> GPMDFVETNSAVYFYGQRDRKFGFLSNFYPCEFTDTEGRRFYSSEQYFMKRKQEMFDRDNEKVAIAILRAKAPAVAKKLGRQVENYDDEVWAEHRYEVMLEALKLKFSSDEEMAAKLLATGAKRLYEASRHDAIWGIGLSVASVTRMFRESVSFQRTGDVDAETRSLCFGKNLLGNALMEARAWLQPQD

Modification of nucleic acids by ADP-ribosylation is catalyzed by various ADP-ribosyltransferases, including the DarT enzyme. The latter is part of the bacterial toxin-antitoxin (TA) system DarTG, which was shown to provide control of DNA replication and bacterial growth as well as protection against bacteriophages. Using structural and biochemical approaches, we show that DarT1-NADAR is a TA system for reversible ADP-ribosylation of guanosine bases. DarT1 evolved the ability to link ADP-ribose to the guanine amino group, which is specifically hydrolyzed by NADAR.

Furthermore, we support our studies with the first crystal structures of NADARs in their ligand-free and ADPr-bound states to structurally characterize the DarT1-associated BC4488 subfamily NADARs in comparison with orphan YbiA subfamily NADARs using that from the plant-pathogenic oomycete Phytophthora nicotianae var. parasitica as an example. The ADPr ligand in the P. nicotianae var. parasitica NADAR crystallographic map displayed a bent binding mode in the open active site, with the protection of its pyrophosphates by the basic side chains of K75 and R79. The adenine head, which directs the N6 amino group toward the active site, is stabilized by π-π interaction with Y84 and hydrogen bonds to K50 and the backbone amides of G78 and V81, the latter water mediated. The adenine-proximal ribose is recognized only by the D86 side chain interacting with the outwards-facing 3′-hydroxyl group, in contrast to the pyrophosphates, which are stabilized by multiple hydrogen bond interactions including K50, R79, W89, R93, W133, and (water-mediated) D130. The distal ribose is coordinated over all three hydroxyl groups, thereby forming either direct (2″) or water-mediated (3″ and 4″) hydrogen bonds to E43 and E125. Interestingly, the corresponding residue in P. nicotianae var. parasitica NADAR (K75) does not directly interact with the ADPr ligand despite being located close to the NADAR active site. To see if the hydrolysis of guanine ADP-ribosylation is a conserved activity of NADAR family members, we tested the non-DarT1-associated NADAR protein of P. nicotianae var. parasitica in the same experimental setup. We observed the reversal of DarT1- and ScARP-catalyzed guanine ADP-ribosylation (Figure 2C lanes 2 and 3) and its inactivity on DarT2-catalyzed thymine ADP-ribosylation modification (Figure 2C lane 1). Since other, non-DarT1-associated and phylogenetically unrelated NADARs such as that in P. nicotianae var. parasitica can also hydrolyze guanine-ADP-ribosyl moieties, this function seems to be evolutionarily conserved among members of different NADAR classes.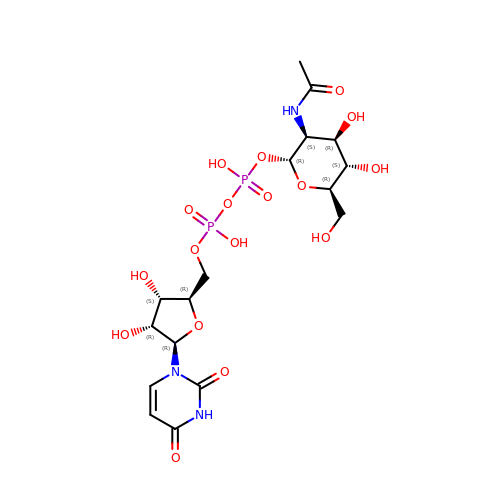(2R,3S,4R,5S,6R)-3-acetamido-4,5-dihydroxy-6-(hydroxymethyl)oxan-2-yl [(2R,3S,4R,5R)-5-(2,4-dioxo-3,4-dihydropyrimidin-1(2H)-yl)-3,4-dihydroxyoxolan-2-yl]methyl dihydrogen diphosphate (non-preferred name) | C17 H27 N3 O17 P2 | LFTYTUAZOPRMMI-ZYQOOJPVSA-N> HYANQLMLSEWLIDVPSDLGQEWIVVVCPVGKRALIVASRGSTSAYTKSGYCVNRFSSLLPGGNRRNSTAKDYTILDCIYNEVNQTYYVLDVMCWRGHPFYDCQ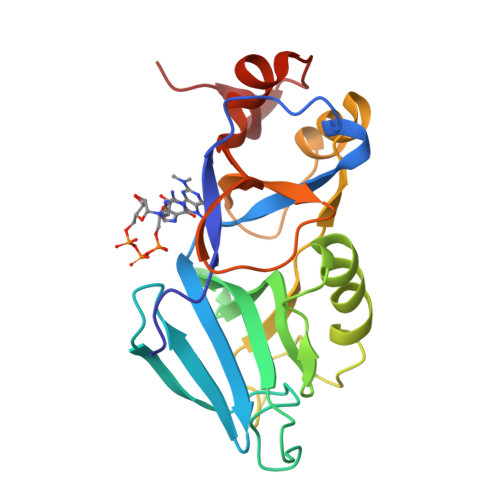TDFRFYWMHSKLPEEEGLGEKTKLNPFKFVGLKNFPCTPESLCDVLSMDFPFEVDGLLFYHKQTHYSPGSTPLVGWLRPYMVSDVLGVAVPAGPLTTKPD> GPGSDAEQRAVAKALFDAVNKHLSNPFIEVEMRLGQFKVEEDANFTACVSTEDYERIKTYLMTEMENSSMTRSVTHDVSLRGWRHTYATDENGNPTRCVSIVRKKRLFVKNIVVPLGAYNLRFAVSTETPGDLRFSGAGPRAGHTRLKDRLSITDGMFRYDMTQVTEKGVLMHEVEIEGVFSSHEKQLTESWLEELLRRAMR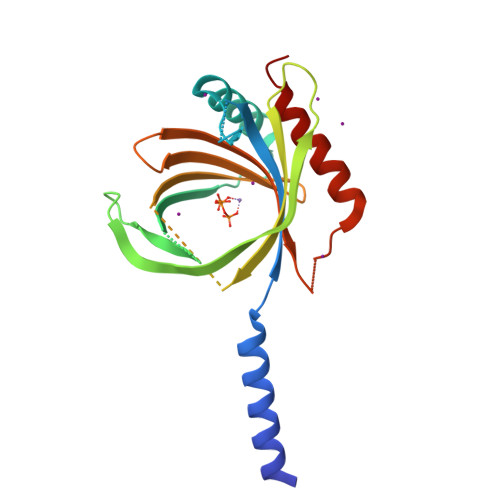LATLRTN>[2x]MGDTKEQRILRYVQQNAKPGDPQSVLEAIDTYCTQKEWAMNVGDAKGQIMDAVIREYSPSL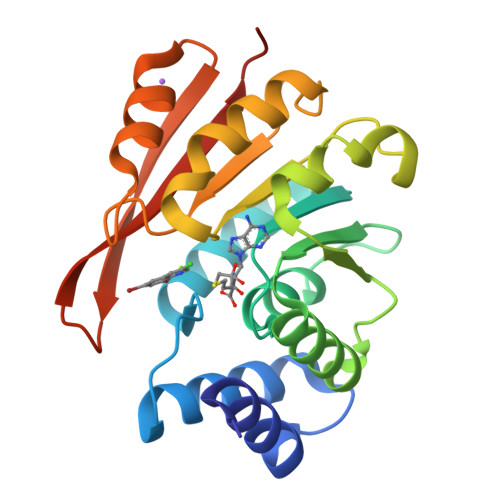VLELGAYCGYSAVRMARLLQPGARLLTMEINPDCAAITQQMLNFAGLQDKVTILNGASQDLIPQLKKKYDVDTLDMVFLDHWKDRYLPDTLLLEKCGLLRKGTVLLADNVIVPGTPDFLAYVRGSSSFECTHYSSYLEYMKVVDGLEKAIYQGPSSPDKS> GPGADRAQDHNNNNTPRNSNYVVEEEEVSEEEEEAIMMPDFGDHVDTSIFGQILEMDEGDDHDFSAPLVLNFFEQAEETFQKMETALNNKDLPELSKLGE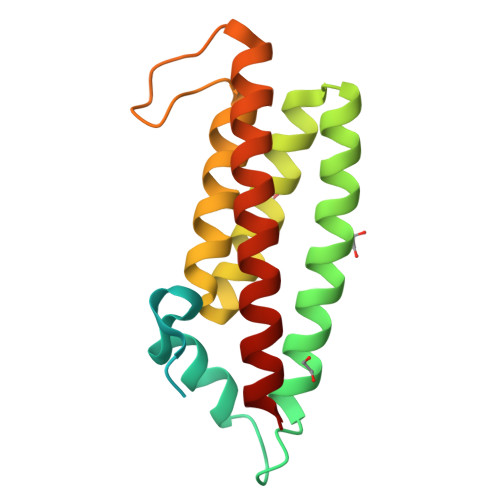FLKGSSATLGFTKIRDSCQLIQQYGHGLNVDGSSEPDEGVCLKKIAEALASARVDTVALHKMMREFFEY>[3x]AQVINTFDGVADYLQTYHKLPDNYITKSEAQALGWVASKGNLADVAPGKSIGGDIFSNRE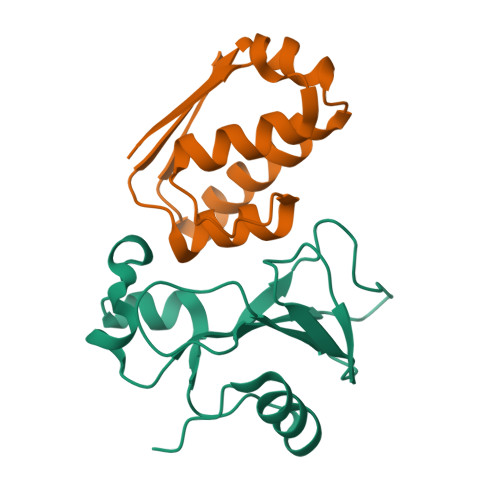GKLPGKSGRTWREADINYTSGFRNSDRILYSSDWLIYKTTDHYQTFTKIR;>KKAVINGEQIRSISDLHQTLKKELALPEYYGENLDALWDALTGWVEYPLVLEWRQFEQSKQLTENGAESVLQVFRAAKAEGADITIILS[3x]Purine nucleoside phosphorylases (PNPs, EC 2.4.2.1) are cytosolic enzymes involved in the purine salvage pathway metabolism in most organisms. The enzyme degrades (2′-deoxy)nucleosides based on 6-oxopurines to the corresponding purine bases and (2-deoxy)ribose-1-phosphate. Purine nucleoside phosphorylase (PNP) is a well-known molecular target with potential therapeutic applications in the treatment of T-cell malignancies and/or bacterial/parasitic infections. The results are supported by a crystallographic study of eight enzyme-inhibitor complexes and by ADMET profiling in vitro and in vivo.

To obtain information on the binding pose and interacting residues, crystal structures of recombinant MtPNP in complex with inhibitors 18c, 45b, and 45q were determined and refined to high resolution. Inhibitors 18c, 45b, and 45q bind to the active site of MtPNP through eight direct and three water-mediated hydrogen bonds. Purine moiety forms direct hydrogen bonds with the sidechains of Glu189, two bonds with Asn231, and a water-mediated bond with the amine group of the Ala234 main chain. Central phenyl moiety interacts with a pocket formed by Tyr188, His243, and Phe153 sidechain belonging to the neighboring molecule within the enzyme trimer. Phosphonate moiety forms five potential direct hydrogen bonds with side chains of Arg88, His90, and Ser208, the main chain of Ser36 and Ala120, and two water-mediated hydrogen bonds with the main chain of Met207 and Tyr180. Positions of purine and phosphonate moieties are identical in all three protein-inhibitor structures, and differences in inhibitor position are observed in the central phenyl moiety. A preliminary in vitro screening revealed that compounds 18b and 18c exhibited low nanomolar inhibitory activities against hPNP (IC50 = 0.021 and 0.022 μM, respectively) and MtPNP (0.025 and 0.031 μM, respectively). All crystallization experiments were performed at 18 °C. The crystal of MtPNP with 18c was obtained using the sitting-drop vapor diffusion technique set by Orynx8 robot (Douglas Instruments) in Swissci 96-well 3-drop plates (Molecular Dimensions). The reservoir solution of 30 μL volume contained 0.2 M magnesium chloride, 30% v/v PEG400, 1 mM Tellurium-Centered Anderson–Evans Polyoxotungstate (TEW), 0.1 M HEPES pH 7.5,54 and drop volume 300 nL, made by mixing equal volumes of the sample and precipitate. Needle crystal, dimensions 300 × 30 × 30 μm appeared after 3 weeks and were harvested after 1 week.

>[3x]VADPRPDPDELARRAAQVIADRTGIGEHDVAVVLGSGWLPAVAALGSPTTVLPQAELPGFVPPTAAGHAGELLSVPIGAHRVLVLAGRIHAYEGHDLRYVVHPVRAARAAGAQIMVLTNAAGGLRADLQVGQPVLISDHLNLTARSPLVGGEFVDLTDAYSPRLRELARQSDPQLAEGVYAGLPGPHYETPAEIRMLQTLGADLVGMSTVHETIAARAAGAEVLGVSLVTNLAAGITGEPLSHAEVLAAGAASATRMGALLADVIARFR>[6x]MRGSHHHHHHGSMDKNIIIGAMTALITPFKNGKVDEQSYARLIKRQIENGIDAVVPVGTTGESATLTHEEHRTCIEIAVETCKGTKVKVLAGAGSNATHAAVGLAKFAKEHGADGILSVAPYYNKPTQQGLYEHYKAIAQSVDIPVLLYNVPGRTGCEISTDTII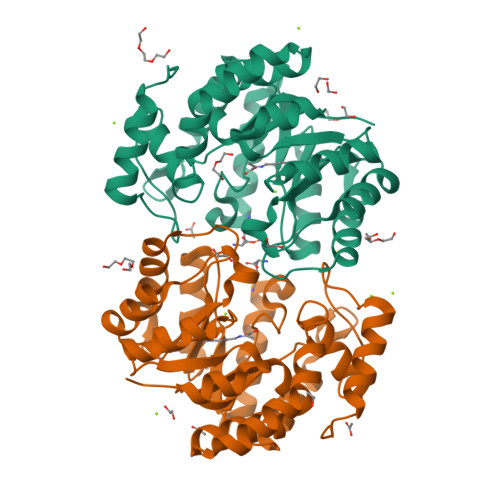KLFRDCENIYGVKEASGNIDKCVDLLAHEPRMMLISGEDAINYPILSNGGKGVISVTSNLLPDMISALTHFALDENYKEAKKINDELYNINKILFCESNPIPIKTAMYLAGLIESLEFRLPLCSPSKENFAKIEEVMKKYKIKGF> MLICKVLKPLVSTNRIPGFEHKHLQVVLDGSSNKVAVDAV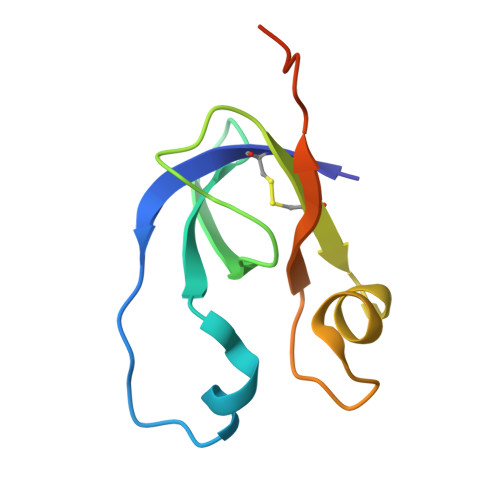GCKPGDWVICVGSSAAREAAGSKSYPSDLTIVGIIDHWDPDSPKQIEV> MECGLNNRIRMIGQICEVAKTKKFEEHAVEALWKAVADLLQPERPLEARHAVLALLKAIVQGQGERLGVLRALFFKVIKDYPSNEDLHERLEVFKALTDNGRHITYLEEELADFVLQWMDVGLSSEFLLVLVNLVKFNSCYLDEYIARMVQMICLLCVRTASSVDIEVSLQVLDAVVCYNCLPAESLPLFIVTLCRTINVKELCEPCWKLMRNLLGTHLGHSAIYNMCHLMEDRAYMEDAPLLRGAVFFVGMALWGAHRLYSLRNSPTSVLPSFYQAMACPNEVVSYEIVLSITRLIKKYRKELQVVAWDILLNIIERLLQQLQTLDSPELRTIVHDLLTTVEELCDQNEFHGSQERYFELVERCADQRPESSLLNLISYRAQSIHPAKDGWIQNLQALMERFFRSESRGAVRIKVLDVLSFVLLINRQFYEEELINSVVISQLSHIPEDKDHQVRKLATQLLVDLAEGCHTHHFNSLLDIIEKVMARSLSPPPELEERDVAAYSASLEDVKTAVLGLLVILQTKLYTLPASHATRVYEMLVSHIQLHYKHSYTLPIASSIRLQAFDFLLLLRADSLHRLGLPNKDGVVRFSPYCVCDYMEPERGSEKKTSGPLSPPTGPPGPAPAGPAVRLGSVPYSLLFRVLLQCLKQESDWKVLKLVLGRLPESLRYKVLIFTSPCSVDQLCSALCSMLSGPKTLERLRGAPEGFSRTDLHLAVVPVLTALISYHNYLDKTKQREMVYCLEQGLIHRCASQCVVALSICSVEMPDIIIKALPVLVVKLTHISATASMAVPLLEFLSTLARLPHLYRNFAAEQYASVFAISLPYTNPSKFNQYIVCLAHHVIAMWFIRCRLPFRKDFVPFITKGLRSNVLLSFDDTPEKDSFRARSTSLNERPKSRIQTSLTSASLGSADENSVAQADDSLKNLHLELTETCLDMMARYVFSNFTAVPKRSPVGEFLLAGGRTKTWLVGNKLVTVTTSVGTGTRSLLGLDSGELQSGPESSSSPGVHVRQTKEAPAKLESQAGQQVSRGARDRVRSMSGGHGLRVGALDVPASQFLGSATSPGP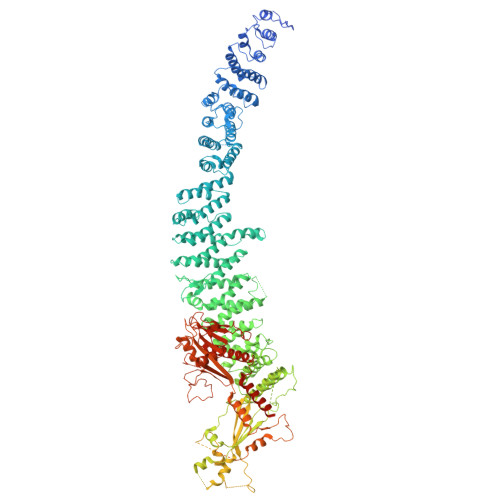RTAPAAKPEKASAGTRVPVQEKTNLAAYVPLLTQGWAEILVRRPTGNTSWLMSLENPLSPFSSDINNMPLQELSNALMAAERFKEHRDTALYKSLSVPAASTAKPPPLPRSNTDSAVVMEEGSPGEVPVLVEPPGLEDVEAALGMDRRTDAYSRSSSVSSQEEKSLHAEELVGRGIPIERVVSSEGGRPSVDLSFQPSQPLSKSSSSPELQTLQDILGDPGDKADVGRLSPEVKARSQSGTLDGESAAWSASGEDSRGQPEGPLPSSSPRSPSGLRPRGYTISDSAPSRRGKRVERDALKSRATASNAEKVPGINPSFVFLQLYHSPFFGDESNKPILLPNESQSFERSVQLLDQIPSYDTHKIAVLYVGEGQSNSELAILSNEHGSYRYTEFLTGLGRLIELKDCQPDKVYLGGLDVCGEDGQFTYCWHDDIMQAVFHIATLMPTKDVDKHRCDKKRHLGNDFVSIVYNDSGEDFKLGTIKGQFNFVHVIVTPLDYECNLVSLQCRKDMEGLVDTSVAKIVSDRNLPFVARQMALHANMASQVHHSRSNPTDIYPSKWIARLRHIKRLRQRICEEAAYSNPSLPLVHPPSHSKAPAQTPAEPTPGYEVGQRKRLISSVEDFTEFV>GSKPFTLPILTLGELSNSRFPVSIDQMYTSPNEVISVQCQNGRCTLDGELQGTTQLQVSGICAFKGEVTAHLQDNGTLYNITITNLNGSPFDPSEDIPAPLGVPDFQGRVFGVITQRDKQNAAGQSQPANRGHDAVVPTYTAQYTPKLGQVQIGTWQTDDLKVNQPVKFTPVGLNDTEHFNQWVVPRYAGALNLNTNLAPSVAPVFPGERLLFFRSYLPLKGGYGNPAIDCLLPQEWVQHF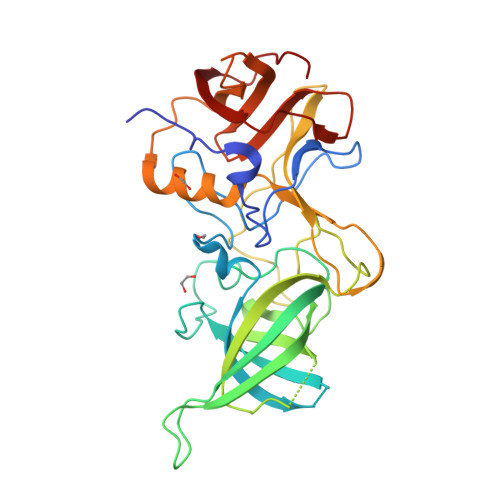YQEAAPSMSEVALVRYINPDTGRALFEAKLHRAGFMTVSSNTSAPVVVPANGYFRFDSWVNQFYSLAPM[3x]> MARSPGRAYALLLLLICFNVGSGLHLQVLSTRNENKLLPKHPHLVRQKRAWITAPVALREGEDLSKKNPIAKIHSDLAEERGLKITYKYTGKGITEPPFGIFVFNKDTGELNVTSILDREETPFFLLTGYALDARGNNVEKPLELRIKVLDINDNEPVFTQDVFVGSVEELSAAHTLVMKINATDADEPNTLNSKISYRIVSLEPAYPPVFYLNKDTGEIYTTSVTLDREEHSSYTLTVEARDGNGEVTDKPVKQAQVQIRILDVNDNIPVVENKVLEGMVEENQVNVEVTRIKVFDADEIGSDNWLANFT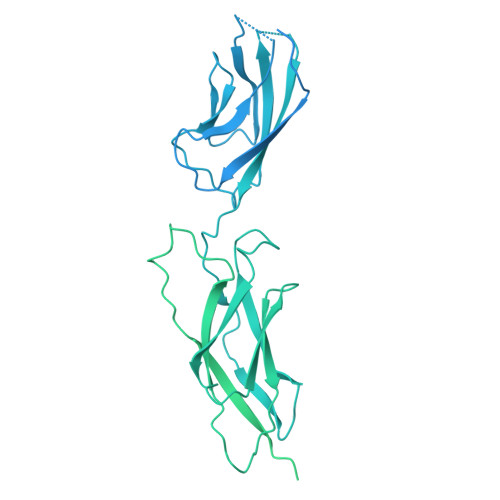FASGNEGGYFHIETDAQTNEGIVTLIKEVDYEEMKNLDFSVIVANKAAFHKSIRSKYKPTPIPIKVKVKNVKEGIHFKSSVISIYVSESMDRSSKGQIIGNFQAFDEDTGLPAHARYVKLEDRDNWISVDSVTSEIKLAKLPDFESRYVQNGTYTVKIVAISEDYPRKTITGTVLINVEDINDNCPTLIEPVQTICHDAEYVNVTAEDLDGHPNSGPFSFSVIDKPPGMAEKWKIARQESTSVLLQQSEKKLGRSEIQFLISDNQGFSCPEKQVLTLTVCECLHGSGCREAQHDSYVGLGPAAIALMILAFLLLLLVPLLLLMCHCGKGAKGFTPIPGTIEMLHPWNNEGAPPEDKVVPSFLPVDQGGSLVGRNGVGGMAKEATMKGSSSASIVKGQHEMSEMDGRWEEHRSLLSGRATQFTGATGAIMTTETTKTARATGASRDMAGAQAAAVALNEEFLRNYFTDKAASYTEEDENHTAKDCLLVYSQEETESLNASIGCCSFIEGELDDRFLDDLGLKFKTLAEVCLGQKIDINKEIEQRQKPATETSMNTASHSLCEQTMVNSENTYSSGSSFPVPKSLQEANAEKVTQEIVTERSVSSRQAQKVATPLPDPMASRNVIATETSYVTGSTMPPTTVILGPSQPQSLIVTERVYAPASTLVDQPYANEGTVVVTERVIQPHGGGSNPLEGTQHLQDVPYVMVRERESFLAPSSGVQPTLAMPNIAVGQNVTVTERVLAPASTLQSSYQIPTENSMTARNTTVSGAGVPGPLPDFGLEESGHSNSTITTSSTRVTKHSTVQHSYS>LPAGCETAILFPMRSKKIFGSVHPVRPMRLESFSACIWVKATDVLNKTILFSYGTKRNPYEIQLYLSYQSIVFVVGGEENKLVAEAMVSLGRWTHLCGTWNSEEGLTSLWVNGELAATTVEMATGHIVPEGGILQIGQEKNGCCVGGGFDETLAFSGRLTGFNIWDSVLSNEEIRETGGAESCHIRGNIVGWGVT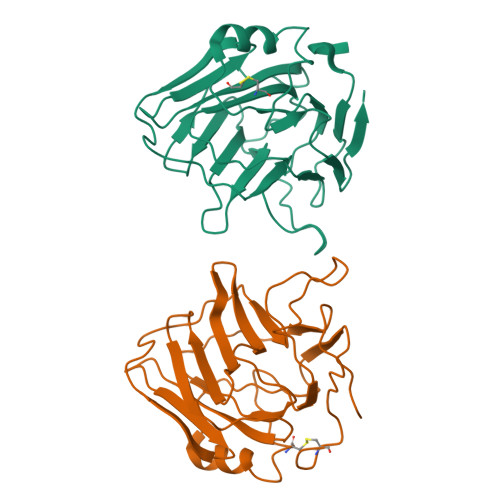EIQPHGGAQYVS[2x]5'-O-[(S)-(carbamoyloxy)(hydroxy)phosphoryl]adenosine | C11 H15 N6 O8 P | 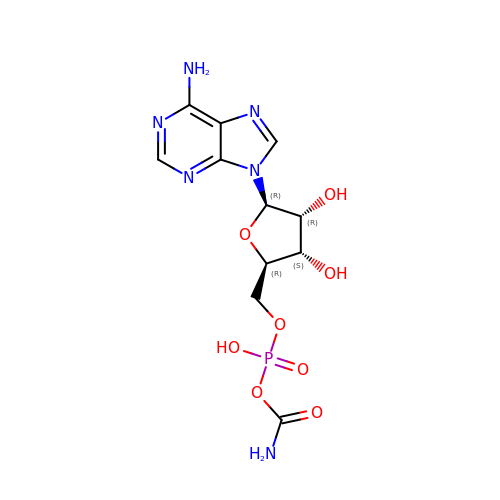CHSNPOFVFYPELH-KQYNXXCUSA-N2-{3-[(2S)-1-acetylpyrrolidin-2-yl]phenyl}-N-(3-chlorophenyl)acetamide 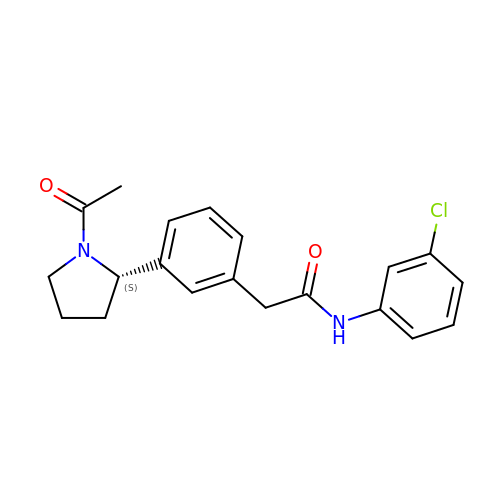| C20 H21 Cl N2 O2 | VRSVKGOGNLDSRR-IBGZPJMESA-N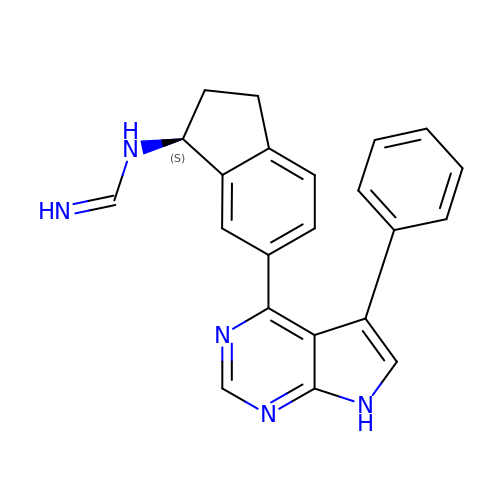N-[(1S)-6-(5-phenyl-7H-pyrrolo[2,3-d]pyrimidin-4-yl)-2,3-dihydro-1H-inden-1-yl]imidoformamide | C22 H19 N5 | HLJVDQSXUUSDJP-IBGZPJMESA-N>GAMALPSGSDPAFSQPKSVLDAGLTCQGASPSSVSKPILLVPGTGTTGPQSFDSNWIPLSAQLGYTPCWISPPPFMLNDTQVNTEYMVNAITTLYAGSGNNKLPVLTVSQGGLVAQWGLTFFPSIRSKVDRLMAFAPDYKGTVLAGPLDALAGSAPSVWQQTTGSALTTALRNAGGLTQIVPTTNLYSATDEIVQPQVSNSPLDSSYLFNGKNVQAQAVCGPLFVIDHAGSLTSQ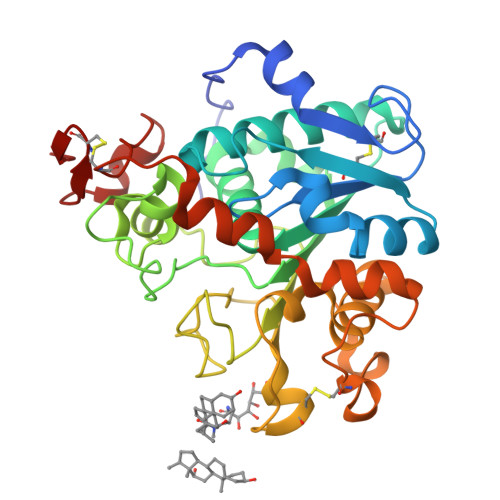FSYVVGRSALRSTTGQARSADYGITDCNPLPANDLTPEQKVAAAALLAPYYAAIVAGPKQNCEPDLMPYARPFAVGKRTCSGIVTP[4x]> GSGSAGSAAGSNHLVKGRSVYELDCIPLWGTVSIQGNRSEMEDAFAVSP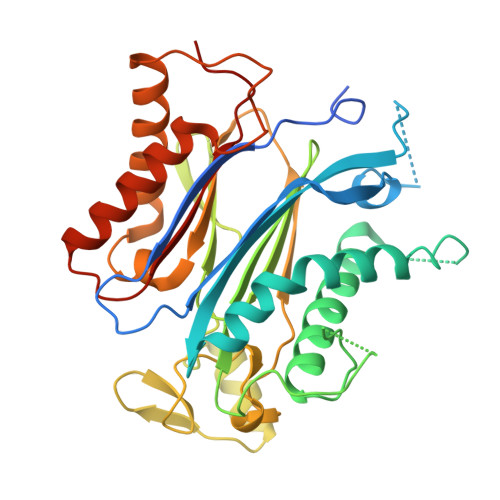HFLKLPIKMLMGDHEGMSPSLTHLTGHFFGVYDGHGGHKVADYCRDRLHFALAEEIERIKDELCKRNTGEGRQVQWDKVFTSCFLTVDGEIEGKIGRAVVGSSDKVLEAVASETVGSTAVVALVCSSHIVVSNCGDSRAVLFRGKEAMPLSVDHKPDREDEYARIENAGGKVIQWQGARVFGVLAMSRSIGDRYLKPYVIPEPEVTFMPRSREDECLILASDGLWDVMNNQEVCEIARRRILMWHKKNGAPPLAERGKGIDPACQAAADYLSMLALQKGSKDNISIIVIDLKAQRKFKTRT>[2x]MSKEYHIDEEVGFALPNPQENLPDFYNDWMFIAKHLPDLIESGQLRERVEKLNMLSIDHLTDHKSQRLARLVLGCITMAYVWGKGHGDVRKVLPRNIAVPYCQLSKKLELPPILVYADCVLANWKKKDPNKPLTYENMDVLFSFRDGDCSKGFFLVSLLVEIAAASAIKVIPTVFKAMQMQERDTLLKALLEIASCLEKALQVFHQIHDHVNPKAFFSVLRIYLSGWKGNPQLSDGLVYEGFWEDPKEFAGGSAGQSSVFQCFDVLLGIQQTAGGGHAAQFLQDMRRYMPPAHRNFLCSLESNPSVREFVLSKGDAGLREAYDACVKALVSLRSYHLQIVTKYILIPASQQPKENKTSEDPSKLEAKGTGGTDLMNFLKTVRSTTEKSLLKEGKGELNSKLEGKPIPNPLLGLDSTRTGHHHHHH

hIDO1 is a heme-containing enzyme that catalyzes the first and rate-limiting step of the kynurenine pathway—the dioxygenation of Trp to N-formyl kynurenine (NFK). It negatively regulates cellular immune response via depleting Trp and promoting the accumulation of kynurenine pathway metabolites. HIDO1 is an α-helical protein, made up by a large C-terminal domain containing the Sa site and a small N-terminal domain sitting on top of it. Here we report the structures of the wild-type hIDO1 in complex with Trp, an inhibitor (epacadostat), and/or an effector (IDE), as well as comparable structures of an active site mutant, F270G.

Trp binding in the Sa site induces the organization of the C-terminal fragment of the highly disordered JK-Loop (referred to as the JK-LoopC hereafter) into a β-hairpin structure, while the N-terminal fragment of the loop (referred to as the JK-LoopN hereafter) unexpectedly remains disordered. The substrate Trp binds in the distal heme pocket, which is enclosed by the JK-LoopC and the DE-Loop, and is capped by a small helix from the N-terminal domain. The binding site is lined with a group of hydrophobic residues, including F226, L234, F163, V130, and Y126. The indole group of the Trp, lying perpendicular to the heme, occupies the so-called “A site”. Its indoleamine group H-bonds with S167 via an intervening water molecule. The ammonium and carboxylate groups extend into the so-called “B site”, forming an interlaced H-bonding network with the conserved “GTGG” motif in the JK-LoopC and the G262 in the DE-Loop, as well as the 7-propionate group of the heme. The carboxylate group is further secured by ion-pairing with R231, which plays a critical role in substrate binding and recognition. Together, these interactions force the iron-bound CN to adopt an unusual bent conformation (with the Fe–C–N angle of ~137°) and position its nitrogen atom next to the C2 atom of the Trp in an oxyanion hole, made up by the indoleamine and ammonium groups of the Trp and the peptide amide group of A264. The active site structure is distinct from that of hTDO, but it resembles that of the hIDO1-O2-Trp complex predicted by QM/MM simulations, offering a direct evidence supporting the hypothesized radical addition mechanism. The Trp-binding site is completely shielded from the bulk solvent, except that a tunnel penetrating from bulk solvent into the distal and proximal heme pockets is evident (displayed as the tint lightblue surface in Fig. 1a).(5R,6R,7R,8S)-7,8-dihydroxy-5-(hydroxymethyl)-5,6,7,8-tetrahydroimidazo[1,2-a]pyridin-6-yl beta-D-glucopyranoside | C14 H22 N2 O9 | 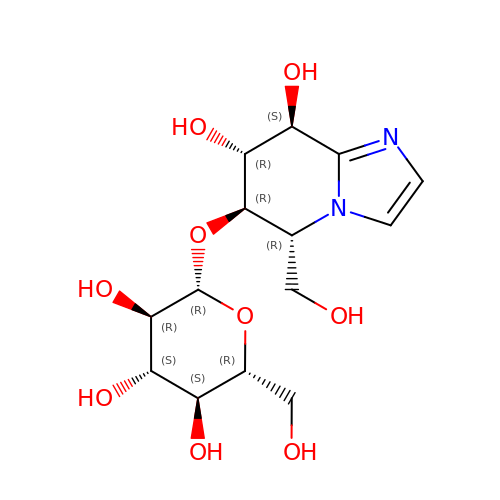CSXOUJBOYXGFCL-OFKZETBZSA-N Replication Protein A (RPA) is a heterotrimeric single stranded DNA-binding protein with essential roles in DNA replication, recombination and repair. In Archaea, the same function is also fulfilled by a heterotrimeric RPA. We report three crystal structures and five cryo-EM structures of Pyrococcus abyssi RPA (hereafter referred to PabRPA), in its apo form as well as bound to ssDNA. We find that archaeal and eukaryotic RPAs share a conserved heterotrimerization core, which is composed of three OB domains connected through a three-helix bundle formed by a C-terminal α-helix from each subunit.

As the use of homopolymeric ssDNA substrates is more convenient for structural studies, we verified that PabRPA binds to a poly-dT ssDNA, with a similar affinity to random ssDNA (1.25 ± 0.6 nM vs 0.71 ± 0.01 nM). Our data show that binding to ssDNA occurs primarily through the Tri-C. Indeed, while a complete PabRPA complex is required for the optimal binding to ssDNA, the Tri-C binds ssDNA with a dissociation constant in the nanomolar range (Kd=18.8 ± 6.0 nM). To gain insights into the structural basis for the high-affinity interaction between PabRPA and ssDNA, we determined the 3.2 Å crystal structure of the Tri-C bound to poly-dT20 ssDNA. The modeled ssDNA lies in a channel that extends from the Rpa1 to the Rpa2 subunits showing 14 contiguous nucleotides that traverse the OB-2 and OB-3 DNA-binding grooves. Rpa3 does not make any contact with the ssDNA in the structure of PabRPA. While both Rpa1 and Rpa2 subunits individually are capable of binding ssDNA, no interaction was observed for the Rpa3 subunit. Indeed, although the chemical nature of the interactions and the overall ssDNA binding path through RPA are conserved, the DNA-binding grooves of the respective OB domains are substantially different in Archaea and Eukarya. In the PabRPA structure, basic residues of the β3-β4 helical insertion in the OB-2 make contact with the DNA phosphodiester backbone and delineate a crevice that is narrower than in the eukaryotic RPA. The helical insertion also exists in eukaryotes but adopts a different conformation and is devoid of conserved basic residues, suggesting that it may be an evolutionary relic derived from an archaeal ancestor. On the other hand, the contacts between the OB-2 Zn-finger domain and ssDNA are remarkably conserved between Archaea and Eukarya. Indeed, in the vicinity of their Zn-finger domains, the interacting residues and the two neighboring bases superimpose perfectly.

> MRISELYPGMDPREVNVVGRVLKKYPPREYTRKDGSVGRVASLIIYDDSGRARVVLWDAKVSEYYNKIEVGDVIKVLDAQVKESLSGLPELHINFRARIILNPDDPRVEMIPPLEEVRVATYTRKKIKDIEAGDRFVEVRGTIAKVYRVLTYDACPECKKKVDYDEGLGVWICPEHGEVQPIKMTILDFGLDDGTGYIRVTLFGDDAEELLGVSPEEIAEKIKELEESGLTTKEAARKLAEDEFYNIIGREIVVRGNVIEDRFLGLILRASSWEDVDYRREIERIKEELEKLGVM;> MSKKRMPATRLYIKDILEGYFVKSEGDFEPNYLITKYARKVYRAKIVGTVVREPLIAEDETYGKFQVDDGTGVIWVLGFRDDTKFAKLVRKGDLVQVIGKIAEWRDDKQILVEGVSKVHPNMWILHRYETLKEKIEHIKKAKIALEIYNQYGITAKSKVIAKNKGIEEELLEVIDELYGIMME;> GTGDGSEVQVRRRKPAVERKISEIREEDTRVSLIGRVIKVDKMDYMFWLDDGTGVAIIESESDLPKVGQVVRVIGRIIRNEEGIHIYAEVIQDFSDADLEALEEIRELERKLLPRLEGEIVW> MVVFNGLLKIKICEAVSLKPTAWSLRDA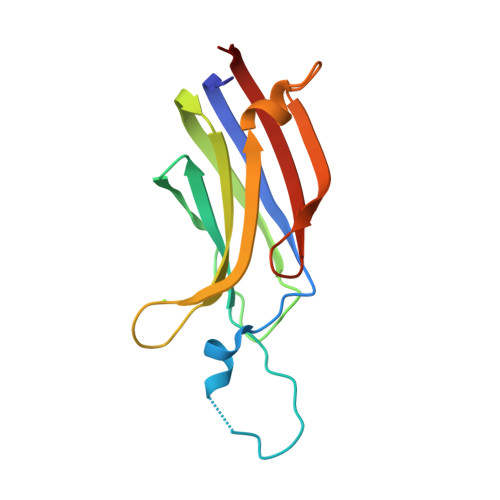VGPRPQTFLLDPYIALNVDDSRIGQTATKQKTNSPAWHDEFVTDVCNGRKIELAVFHDAPIGYDDFVANCTIQFEELLQNGSRHFEDWIDLEPEGKVYVIIDLSGSSG>[2x]SELKQAFVFEFDENLSSSSGSIHLEKVKQNSSPNYDYFKITFIDGYLYIKNKSGVILDKYDLKNVISLVALKRDYLSLSLSNNKQIKKFKNIKNKHLKNKFNLYVINEDIEK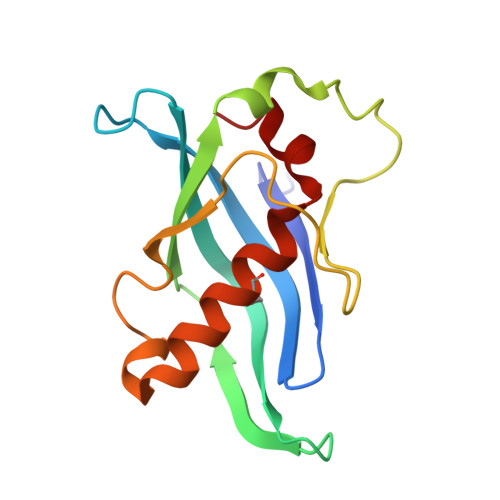RITKNGILEEVILNKMLLSILLGNEENLLQIS(4R)-1-methyl-4-(prop-1-en-2-yl)cyclohex-1-ene 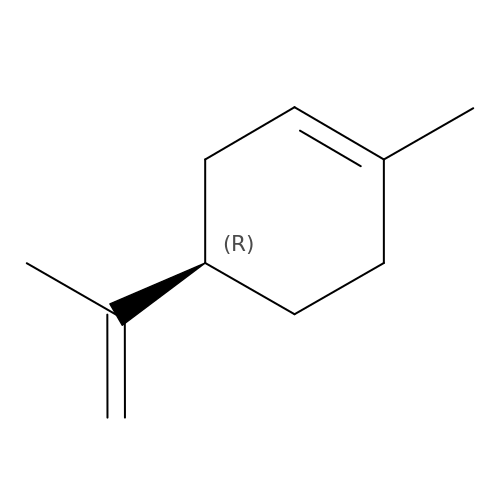| C10 H16 | XMGQYMWWDOXHJM-JTQLQIEISA-N>[2x]MSLLKIYWRAMQYLAVERTATITMCVASVLVALVTLAEPVLFGRVIQSISDKGDIFSPLLMWAALGGFNIMAAVFVARGADRLAHRRRLGVMIDSYERLITMPLAWHQKRGTSNALHTLIRATDSLFTLWLEFMRQHLTTVVALATLIPVAMTMDMRMSLVLIVLGVIYVMIGQLVMRKTKDGQAAVEKHHHKLFEHVSDTISNVSVVQSYNRIASETQALRDYAKNLENAQFPVLNWWALASGLNRMASTFSMVVVLVLGAYFVTKGQMRVGDVIAFIGFAQLMIGRLDQISAFINQTVTARAKLEEFFQMEDATADRQEPENVADLNDVKGDIVFDNVTYEFPNSGQGVYDVSFEVKPGQTVAIVGPTGAGKTTLINLLQRVFDPAAGRIMIDGTDTRTVSRRSLRHAIATVFQDAGLFNR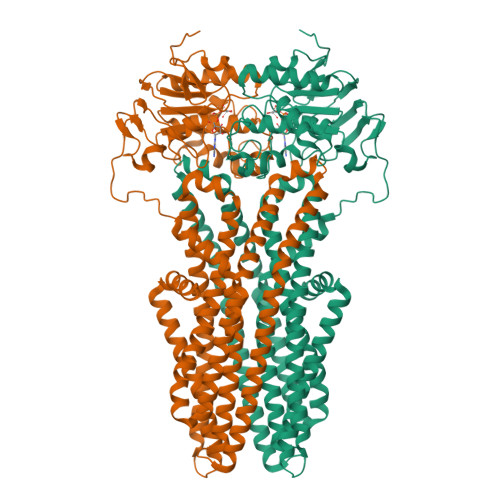SVEDNIRVGRANATHEEVHAAAKAAAAHDFILAKSEGYDTFVGERGSQLSGGERQRLAIARAILKDSPILVLDEATSALDVETEEKVTQAVDELSHNRTTFIIAHRLSTVRSADLVLFMDKGHLVESGSFNELAERGGRFSDLLRAGGLKLEDKQPKQPVVEGSNVMPFPVKGAVA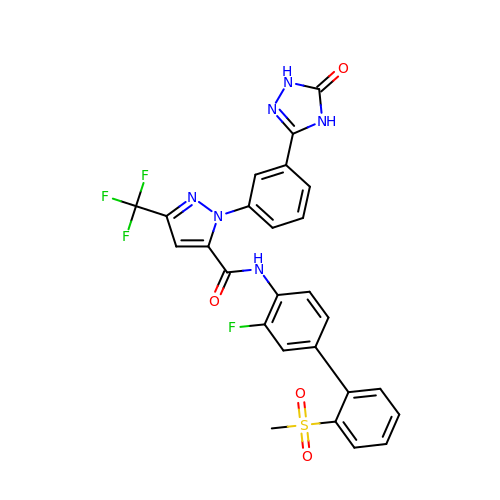N-(3-FLUORO-2'-(METHYLSULFONYL)BIPHENYL-4-YL)-1-(3-(5-OXO-4,5-DIHYDRO-1H-1,2,4-TRIAZOL-3-YL)PHENYL)-3-(TRIFLUOROMETHYL)-1H-PYRAZOLE-5-CARBOXAMIDE | C26 H18 F4 N6 O4 S | YIHPFOJBRPDMES-UHFFFAOYSA-N> MAHHHHHHMLKLIVETKTLVQSLGFASSVVEKRNVIPEYANIKLSAQDGNLELSSTNMDLYLSQKIAVQVVSEGECTVSTKTLNDIVRKLPDSELTLTDLGTTGLEIKGKNCKFNLFTLPVSSFPAMDSINPEASFKISCTDFAKIIESTKFSISLDETRYNLNGVYLHIKDKEFCSASTDGHRLSISWVTLEKQIKNFGVILPQKSAEE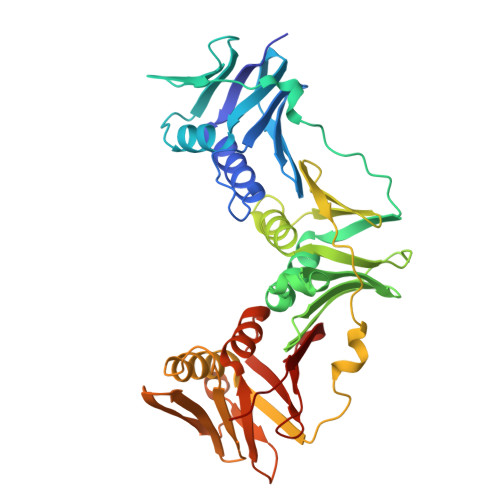ILKIVKDPKNINEDIEILLNSNKIKFICNENTIMLSKLIDGTFPDYSTFIPESSSSKLVINRKMFADSIERIAIITVEKFRAVKLSLSRETLEISAVGEARGNAKEVINSSQDKESFYEYNSDESLAIGFNPQYLEDVLKAVKSDLVELYFSDVSAPVLIKFPENPKDIFIVLPVKV> MATDVAQGPNGRALAESMNPDLLSAIQQHISIERYASVTYLAMSIWCAERELAGFYQFFDGEAKAEQSHAVHFTQYLIARSQSNDLQTLDAPRQNWDSLASLMATAFQMEADTTSSIQSVYALAERNSDTRTTVFLDPLIEAQIQSEDQFAYLLGRVKFANGDPTALLVIDNELRAGQTQRG

Ferritins are proteins forming 24meric rhombic dodecahedral cages that play a key role in iron storage and detoxification in all cell types. Their function requires the transport of Fe2+ from the exterior of the protein to buried di-iron catalytic sites, known as ferroxidase centres, where Fe2+ is oxidized to form Fe3+-oxo precursors of the ferritin mineral core. SynFtn, isolated from the cyanobacterium Synechococcus CC9311, is an atypical prokaryotic ferritin that was recently shown to take up Fe2+ via its threefold channels. The wild-type protein contains three iron binding sites: high- and low-affinity binding sites at the FOC, sites 1 and 2, respectively, and site 3 located in the threefold channel and coordinated by the side chains of three symmetry equivalent Asp137 residues.

High-resolution structures of SynFtn revealed that the side chain of residue Asp65 lies in close proximity to Glu62, raising the possibility that the two residues form a transient binding site for iron. Variant D65A was therefore constructed to determine the importance of this residue in SynFtn function. Variant D65A also crystallized under identical conditions to those reported for wild-type SynFtn, and the resulting D65A structure overlays with that for the wild-type protein (overall rmsd of 0.09 Å). Protein structures derived from all crystals harvested without iron enrichment were free of bound metal ions, as expected. In the metal-free structure of variant D65A the side chain of Glu141 is oriented towards the threefold channel, and, in contrast to wild-type protein, the exposure of crystals to Fe2+ for either 2 or 20 min did not lead to a change in conformation of Glu141, regardless of the fractional occupancy of site 3. However, the rate at which Fe2+ binds to FOC sites in variant D65A was only 50 % that of the wild-type protein under the same conditions, suggesting a role for Asp65 in uptake of Fe2+. In contrast, the initial rate of mineral core formation in variant D65A is 0.35 µm s−1, only ~35 % of the 0.95 µm s−1 rate of wild-type SynFtn, consistent with the hypothesis that Asp65 plays a role in transporting ferric-oxo species away from the FOC. Therefore, the impaired mineralization activity of variant D65A cannot be a consequence of increased stability of the di-Fe3+ form of the FOC, as was reported for variant E62A, suggesting that the replacement of Asp65 has a less direct effect on the exit of Fe3+ from the FOC. In the absence of Asp65, the pathway for Fe2+ into the FOC may be altered, apparently resulting in inhibition of Fe3+ egress, and suggesting that the pathways for iron entry and exit from the FOC are closely associated, such that disruption of the uptake route can cause a clash with the exit route.>[3x]MSSNPLRFFVLTIFPHIISCYSEYGIVKQAIKKGKVEVYPIDLREFAPKGQVDDVPYGGLPGMVLKPEPIYEAYDYVVENYGKPFVLITEPWGEKLNQKLVNELSKKERIMIICGRYEGVDERVKKIVDMEISLGDFILSGGEIVALAVIDAVSRVLPGVLSEPQSIQEDSFQNRWLGYPVYTRPREYRGMKVPEELLSG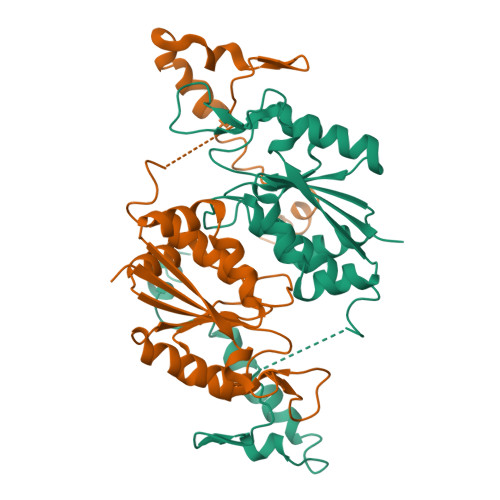HHKLIELWKLWHRIENTVKKRPDLIPKDLTELEKDILNSILSGKSFKEWLKEHKHLL2,2,4,4,6,6,8-heptamethylnonane | C16 H34 | 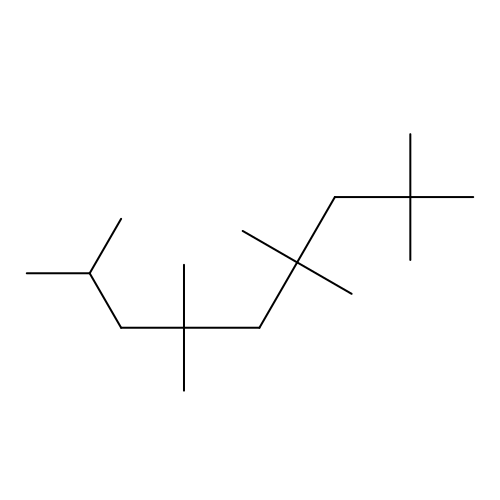RDUBCTHNBWFPTP-UHFFFAOYSA-N>MAAKLWTFLLGFGLSWVWPASAHRKLLVLLLDGFRSDYISEDALASLPGFREIVNRGVKVDYLTPDFPSLSYPNYYTLMTGRHCEVHQMIGNYMWDPRTNKSFDIGVNRDSLMPLWWNGSEPLWITLMKARRKVYMYYWPGCEVEILGVRPTYCLEYKTVPTDINFANAVSDALDSLKSGRADLAAIYHERIDVEGHHYGPSSPQRKDALRAVDTVLKYMIQWIQDRGLQQDLNVILFSDHGMTDIFWMDKVIELSNYISLDDLQQVKDRGPVVSLWPVPGKHSEIYHKLRTVEHMTVYEKESIPNRFYYKKGKFVSPLTLVADEGWFIAESREMLPFWMNSTGKREGWQRGWHGYDNELMDMRGIFLAIGPDFKSNFRAAPIRSVDVYNIMAHVAGITPLPNNGSWSRVVSMLKGQTSSASRENLYFQ[2x]

The ecto-nucleotide pyrophosphatases/phosphodiesterases (ENPPs or NPPs) family consists of seven structurally-related ecto-enzymes. ENPP6 hydrolyzes only choline-containing lysophospholipids, such as LPC, sphingosylphosphorylcholine (SPC), platelet-activating factor (PAF) and lysoPAF, but not other lysophospholipids, suggesting that ENPP6 recognizes the choline moiety of its substrates. Here, we showed that GPC is hydrolyzed to phosphocholine by ENPP6, which is present on the extracellular surface of certain cells such as oligodendrocytes and liver sinusoid endothelial cells. In addition, we showed that ENPP6-deficient mice have impaired myelin structure and are prone to having a fatty liver, which are typical symptoms of choline deficiency. Together, these results strongly suggest that ENPP6 serves as a choline-supplying enzyme.

Accordingly, we also determined the crystal structure of ENPP6 in complex with phosphocholine, a reaction product, at 1.8 Å resolution. An electron density corresponding to the bound phosphocholine was observed in the vicinity of the zinc ions in the catalytic pocket. The choline moiety of the phosphocholine is accommodated in a choline-binding pocket formed by the side chains of Tyr72, Tyr75, Tyr157 and Tyr188, while the phosphate group of the phosphocholine is located in the vicinity of the two zinc ions. Tyr72, Tyr75 and Tyr188 provide π-cation interactions with the positively-charged choline moiety. Furthermore, Asp32 and Glu190 electrostatically interact with the choline moiety. Tyr72 forms a water-mediated hydrogen bond with Glu143, while Tyr75/Tyr188 and Tyr157 form direct hydrogen bonds with Asp32 and Glu190, respectively, thereby stabilizing the conformation of the choline-binding pocket. In addition, Trp139 and Pro140 in the “insertion loop” (residues 139–157) interact with the side chains of Tyr72, Tyr75, Tyr157 and Tyr188. The conformation of the “insertion loop” is stabilized by a disulfide linkage between Cys142 and Cys154. The Y72A, Y75A, Y188A and E190A mutants exhibited the remarkably reduced α-GPC-hydrolyzing activities, as compared with the wild-type and C393A/C412S mutant proteins, confirming the importance of Tyr72, Tyr75, Tyr188 and Glu190 for choline recognition. The crystal structure of the ENPP6–phosphocholine complex showed that ENPP6 recognizes the choline moiety of phosphocholine, which strongly supports the idea that ENPP6 recognizes the choline moiety of its substrates, such as GPC and LPC, and hydrolyzes them to produce phosphocholine in a similar manner.3-(5-bromo-1H-indol-3-yl)-2-thioxopropanoic acid | C11 H8 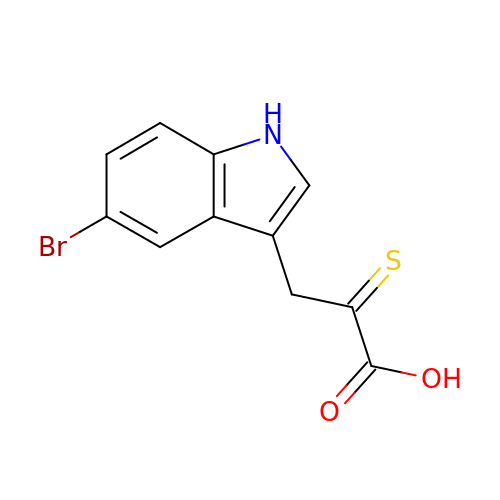Br N O2 S | XFDKQHURWNNDLG-UHFFFAOYSA-N The SF3b core complex contains several spliceosome-associated proteins (SAPs), including SF3B1/SAP155, SF3B2/SAP145, SF3B3/SAP130, SF3B4/SAP49, SF3B5/SAP10, SF3B6/SAP14a and PHF5A/SAP14b. Here, by integrating structural and biochemical approaches with a modified chemogenomic strategy utilizing structurally different splicing modulators at permissive dosage for resistant mutation(s) mapping, we report that PHF5A, a core component of the SF3b complex, is a common cellular target of splicing-modulating chemical probes, including herboxidiene, pladienolide, spliceostatin and sudemycin. The full-length Rds3 protein was recently observed in the cryo-EM structure of the spliceosome Bact complex at a resolution range of 3.0–3.5 Å15. This structure shows that Rds3/PHF5A is a central scaffolding protein, interacting with Hsh155/SF3B1, Rse1/SF3B3, Ysf3/SF3B5, U2 snRNA and the intron RNA. In summary, we identify PHF5A as a key node of interaction for small-molecule splicing modulators.

We purified the WT protein and determined the crystal structure at 1.8 Å resolution. Our final model contains residues 2–93 out of 110 total. PHF5A forms a mushroom-like structure with a triangular-shaped cap and a stem composed of antiparallel strands from the N and C termini. The cap is formed by a left-handed, triangular, deep trefoil knot containing three zinc ions and five CXXC motifs, which are permuted between the zinc fingers. PHF5A contains 13 Cys residues and 12 of these coordinate 3 zinc ions in tetrahedral geometry. The remaining cysteine was mutated to serine (C40S) to enhance soluble protein expression. Interestingly, PHF5A incorporates three different types of zinc finger. Zinc-finger 1 (ZnF1) folds into a gag knuckle and has C4 coordination from the first and fourth CXXC motifs. Zinc-finger 2 (ZnF2) is formed by the second and fifth CXXC motifs. Zinc-finger 3 (ZnF3) is formed by the third CXXC motif from helix-η2 and two individual cysteines from the loops connecting the first and the last beta strands of the mushroom stem.

>[2x]GGHMAKHHPDLIFCRKQAGVAIGRLCEKCDGKCVICDSYVRPSTLVRICDECNYGSYQGRCVICGGPGVSDAYYCKECTIQEKDRDGCPKIVNLGSSKTDLFYERKKYGFKKR> CPEQDKYRTITGMCNNRRSPTLGASNRAFVRWLPAEYEDGFSLPYGWTPGVKRNGFPVALARAVSNEIVRFPTDQLTPDQERSLMFMQWGQLLDHDLDFTPEPAARASFVTGVNCETSCVQQPPCFPLKIPPNDPRIKNQADCIPFFRSCPACPGSNITIRNQINALTSFVDASMVYGSEEPLARNLRNMSNQLGLLAVNQRFQDNGRALLPFDNLHDDPCLLTNRSARIPCFLAGDTRSSEMPELTSMHTLLLREHNRLATELKSLNPRWDGERLYQEARKIVGAMVQIITYRDYLPLVLGPTAMRKYLPTYRSYNDSVDPRIANVFTNAFRYGHTLIQPFMFRLDNRYQPMEPNPRVPLSRVFFASWRVVLEGGIDPILRGLMATPAKLNRQNQIAVDE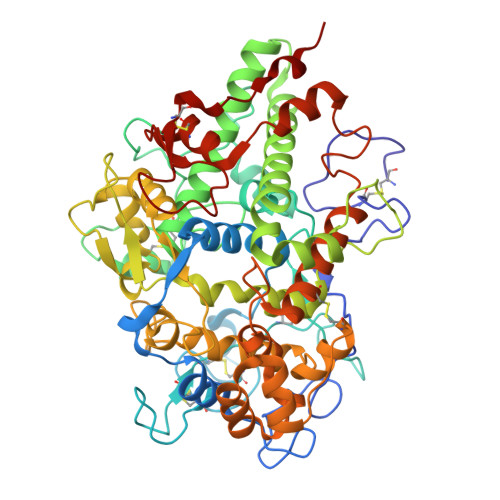IRERLFEQVMRIGLDLPALNMQRSRDHGLPGYNAWRRFCGLPQPETVGQLGTVLRNLKLARKLMEQYGTPNNIDIWMGGVSEPLKRKGRVGPLLACIIGTQFRKLRDGDRFWWENEGVFSMQQRQALAQISLPRIICDNTGITTVSKNNIFMSNSYPRDFVNCSTLPALNLASWREA> MGHHHHHHS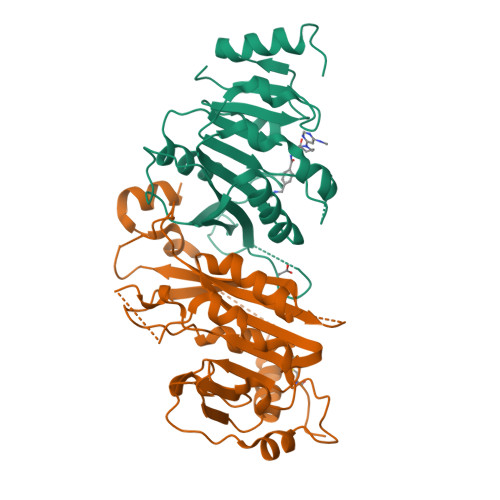SGRENLYFQGALTQSVGGDSSADRLFPPQWICCDIRYLDVSILGKFAVVMADPPWDIHMELPYGTLTDDEMRRLNIPVLQDDGFLFLWVTGRAMELGRECLNLWGYERVDEIIWVKTNQLQRIIRTGRTGHWLNHGKEHCLVGVKGNPQGFNQGLDCDVIVAEVRSTSHKPDEIYGMIERLSPGTRKIELFGRPHNVQPNWITLGNQLDGIHLLDPDVVARFKQRYPDGIISKPKNL;> MLKGTQSLNPHNDYCQHFVDTGHRPQNFIRDVGLADRFEEYPKLRELIRLKDELIAKSNTPPMYLQADIEAFDIRELTPKFDVILLEPPLEEYYRETGITANEKCWTWDDIMKLEIDEIAAPRSFIFLWCGSGEGLDLGRVCLRKWGYRRCEDICWIKTNKNNPGKTKTLDPKAVFQRTKEHCLMGIKGTVKRSTDGDFIHANVDIDLIITEEPEIGNIEKPVEIFHIIEHFCLGRRRLHLFGRDSTIRPGWLTVGPTLTNSNYNAETYASYFSAPNSYLTGCTEEIERL> MHHHHHHMKSIDEQSLHNARRLFESGDIDRIEVGTTAGLQQIHRYLFGGLYDFAGQIREDNISKGGFRFANAMYLKEALVKIEQMPERTFEEIIAKYVEMNIAHPFLEGNGRSTRIWLDLVLKKNLKKVVNWQNVSKTLYLQAMERSPVNDLELRF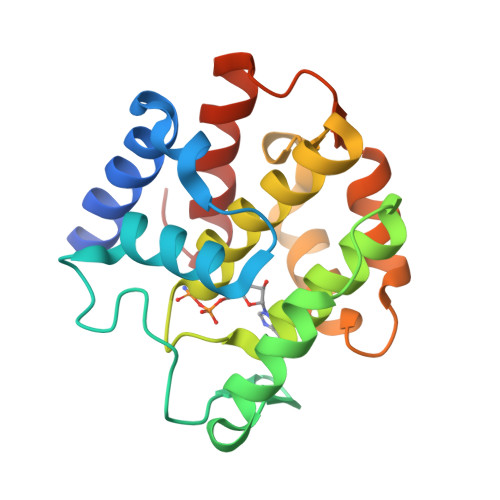LLKDNLTDDVDNREIIFKGIEQSYYYEGYEKG The EphA4 tyrosine kinase cell surface receptor regulates an array of physiological processes and is the only currently known class A Eph receptor that binds both A and B class ephrins with high affinity. Eph receptors are type 1 membrane proteins with an N-terminal extracellular region consisting of a ligand binding domain (LBD), a cysteine rich region, and two fibronectin type III domains. We have solved the crystal structure of the EphA4 ligand binding domain alone and in complex with (1) ephrinB2 and (2) ephrinA2. Structural analyses, drawing on previously reported Eph receptor structures, show that EphA4 in isolation and in complex with ephrinA2 resembles other class A Eph receptors but on binding ephrinB2 assumes structural hallmarks of the class B Eph receptors. This interactive plasticity reveals EphA4 as a structural chameleon, able to adopt both A and B class Eph receptor conformations, and thus provides a molecular basis for EphA-type cross-class reactivity.

The EphA4-ephrinB2 structure is the first cross-class EphA type complex. In the EphA4-ephrinB2 structure, electron density corresponding to a single N-acetylglucosamine moiety was observed at Asn36ephrinB2 (conserved with Asn42ephrinA2) but not Asn139ephrinB2. In contrast, the JKEphA4 loop is very different between its two bound states (2.8 Å rmsd over Cα atoms of residues Ala150EphA4-Leu166EphA4); forming an extended conformation when bound to ephrinB2 and an α helix (Gln156EphA4-Asp161EphA4) when bound to ephrinA2. The extended conformation of the JKEphA4 loop when bound to ephrinB2 appears to be stabilized by a hydrophobic stacking interaction between Arg162EphA4 and Trp122ephrinB2 (Trp122 is equivalent to Trp125 in mouse). As a result, we suggest that the plasticity of the JKEphA4 loop region allows EphA4 to physically adapt to Trp122ephrinB2 and the resulting complementary stacking interactions with Arg162EphA4 are compensatory. While the EphA4-ephrinB2 interface is comprised of 15 hydrogen bonds and a total of 30 residues participating in van der Waals interactions, EphA4-ephrinA2 contains only 6 and 22, respectively. Conspicuously, in the Eph receptor tree, EphA4 in its ephrinB2-bound state is the most structurally similar out of all A class Eph receptors to the B class Eph receptors. It appears that EphA4 maintains an element of conformational duality and flexibility that allows it to act as a pseudo class B Eph receptor, but, in corroboration with our surface plasmon resonance binding data, at an energetic cost with reduced binding affinity. We find that EphA4 has greatest affinity for ephrinA4 (KD = 36 nM), intermediate affinities to ephrinA1, ephrinA5, and ephrinA2 (KD = 1.2 μM, KD = 360 nM, and KD = 2.3 μM, respectively), binds most weakly to ephrinB2 (KD = 10.8 μM), and shows no detectable binding to ephrinB1.

> ETGEVTLLDSRSVQGELGWIASPLEGGWEEVSIMDEKNTPIRTYQVCNVMEPSQNNWLRTDWITREGAQRVYIEIKFTLRDCNSLPGVMGTCKETFNLYYYESDNDKERFIRENQFVKIDTIAADESFTQVDIGDRIMKLNTEIRDVGPLSKKGFYLAFQDVGACIALVSVRVFYKRTKHHHHHH;> ETGSIVLEPIYWNSSNSKFLPGQGLVLYPQIGDKLDIICPKVDSKTVGQYEYYKVYMVDKDQADRCTIKKENTPLLNCAKPDQDIKFTIKFQEFSPNLWGLEFQKNKDYYIISTSNGSLEGLDNQEGGVCQTRAMKILMKVGQDGTKHHHHHH> MEKGDTHILVFPFPAQGHINPLLQLSKHLIAKGIKVSLVTTLHVSNRMQLQGAYSNSVKIEVISDGSEDRLETDTLRQYLDRFRQKMTKNLEDFLQKAMVSSNPPKFIIYDSTMPWVLEVAKEFGLDRAPFYTQSCALNSINYHVLHGQLKLPPETPTISLPSMPLLRPSDLPAYDFDPASTDTIIDLLTSQYSNIQDANLLFCNTFDKLEGEIIQWMETLGRPVKTVGPTVPSAYLDKRVENDKHYGLSLFKPNEDVCLKWLDSKPSGSVLYVSYGSLVEMGEEQLKELALGIKETGKFFLWVVRDTEAEKLPPNFVESVAEKGLVVSWCSQLEVLAHPSVGCFFTHCGWNSTLEALCLGVPVVAFPQWADQVTNAKFLEDVWKVGKRVKRNEQRLASK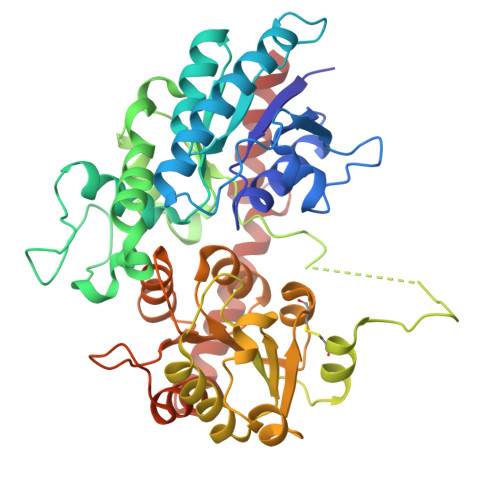EEVRSCIWEVMEGERASEFKSNSMEWKKWAKEAVDEGGSSDKNIEEFVAMLKQT>MSSILRLDRLRQFIGELATLLDSRPDESTLLAQAHPLLAELVHQDDWLPEDCARPDPQRYQQYLLHVDSRQRFSVVSFVWGPGQITPVHDHRVWCLIGMLRGAEYSQPYAFDAGGRPHPSGARRRLEPGEVEALSPRIGDVHQVSNAFSDRTSISIHVY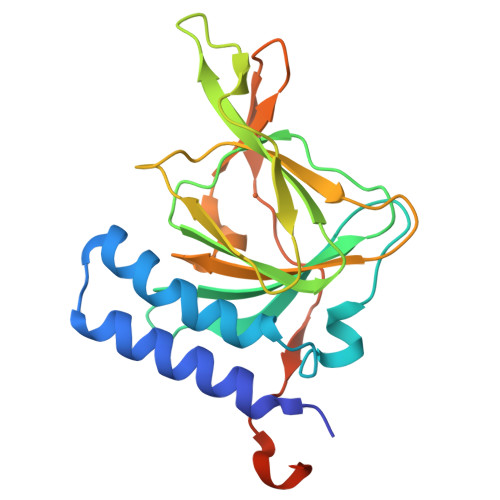GANIGAVRRAVFSAEGEEKPFISGYSNSRLPNIWDLSKENPASAWSHPQFEK[4x]>[2x]GHHHHHHHHHHSSGHIEGRHMRVLFVSSPGIGHLFPLIQLAWGFRTAGHDVLIAVAEHADRAAAAGLEVVDVAPDYSAVKVFEQVAKDNPRFAETVATRPAIDLEEWGVQIAAVNRPLVDGTMALVDDYRPDLVVYEQGATVGLLAADRAGVPAVQRNQSAWRTRGMHRSIASFLTDLMDKHQVSLPEPVATIESFPPSLLLEAEPE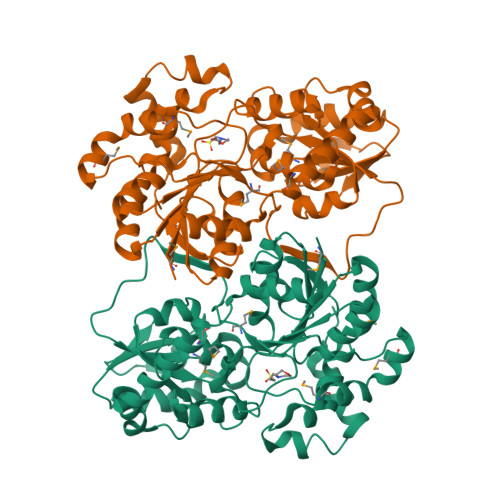GWFMRWVPYGGGAVLGDRLPPVPARPEVAITMGTIELQAFGIGAVEPIIAAAGEVDADFVLALGDLDISPLGTLPRNVRAVGWTPLHTLLRTCTAVVHHGGGGTVMTAIDAGIPQLLAPDPRDQFQHTAREAVSRRGIGLVSTSDKVDADLLRRLIGDESLRTAAREVREEMVALPTPAETVRRIVERISG> MVSVSEIRKAQRAEGPATILAIGTANPANCVEQSTYPDFYFKITNSEHKTELKEKFQRMCDKSMIKRRYMYLTEEILKENPNVCEYMAPSLDARQDMVVVEVPRLGKEAAVKAIKEWGQPKSKITHLIVCTTSGVDMPGADYQLTKLLGLRPYVKRYMMYQQGCFAGGTVLRLAKDLAENNKGARVLVVCSEVTAVTFRGPSDTHLDSLVGQALSGD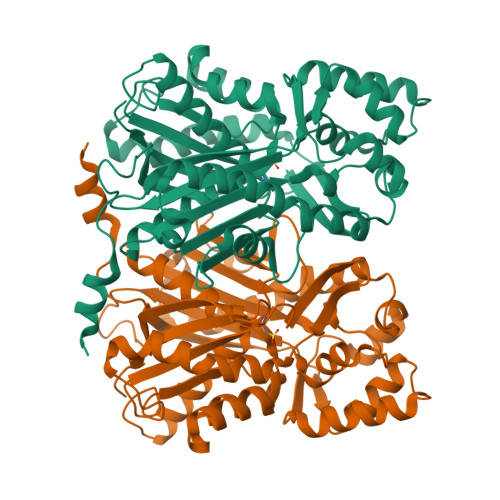GAAALIVGSDPVPEIEKPIFEMVWTAQTIAPDSEGAIDGHLREAGLTFHLLKDVPGIVSKNITKALVEAFEPLGISDYNSIFWIAHPGGPAILDQVEQKLALKPEKMNATREVLSEYGNMSSACVLFILDEMRKKSTQNGLKTTGEGLEWGVLFGFGPGLTIETVVLRSVAI(4~{S})-4-(4-chloranyl-2-methyl-phenyl)-5-(5-chloranyl-2-methyl-phenyl)-2-(2,4-dimethoxypyrimidin-5-yl)-3-propan-2-yl-4~{H}-pyrrolo[3,4-d]imidazol-6-one 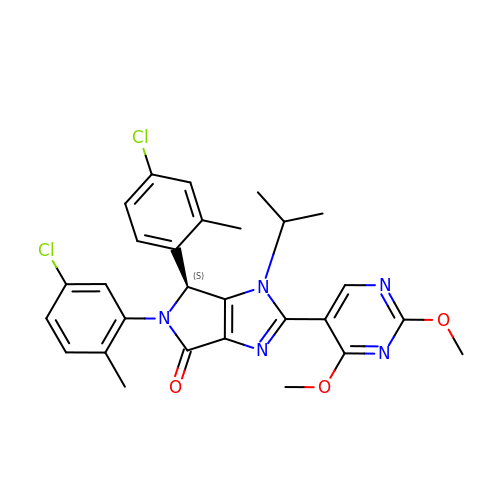| C28 H27 Cl2 N5 O3 | XBJHBEQDHSREQB-QHCPKHFHSA-N> QDNSRYTHFLTQHYDAKPQGRDDRYCESIMRRRGLTSPCKDI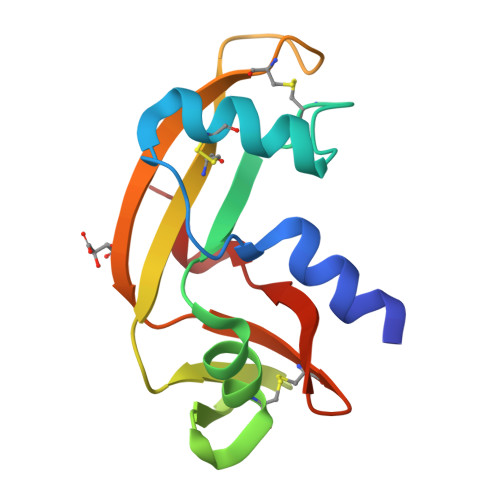NTFIHGNKRSIKAICENKNGNPHRENLRISKSSFQVTTCKLHGGSPWPPCQYRATAGFRNVVVACENGLPIHLDQSIFRRP> ELQKSIGKKPEPTDEEWELIKTVTEAHVATNAQGSHWKQKRKFLPEDIGQAPIVNAPEGGKVDLEAFSHFTKIITPAITRVVDFAKKLPMFCELP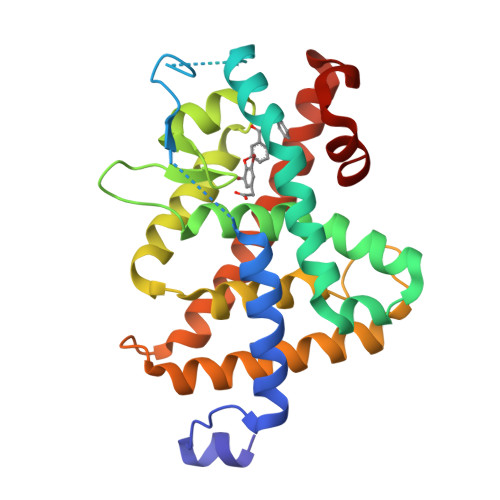CEDQIILLKGCCMEIMSLRAAVRYDPESETLTLNGEMAVTRGQLKNGGLGVVSDAIFDLGMSLSSFNLDDTEVALLQAVLLMSSDRPGLACVERIEKYQDSFLLAFEHYINYRKHHVTHFWPKLLMKVTDLRMIGACHASRFLHMKVECPTELFPPLFLEVFED The bacterial injectisome, or type III secretion system (T3SS), is a specialized syringe-shaped protein-export system utilized by many pathogenic Gram-negative bacteria for the injection of virulence proteins (effectors) into host cells. The injectisome can be divided into three major regions: the inner- (IM) and outer-membrane (OM) spanning basal body with associated export apparatus and ATPase components, an extracellular needle, and a terminating pore inserted into the host cell membrane called the translocon. The major structural scaffold of the basal body is comprised largely of three proteins that arrange into a series of highly oligomerized, concentric rings: two intimately associated proteins localized to the IM - PrgK/EscJ/MxiJ and PrgH/EscD/MxiG, and a third protein belonging to the secretin family of OM proteins, InvG/EscC/MxiD (Salmonella enterica serovar Typhimurium SPI-1, Enteropathogenic Escherichia coli (EPEC) LEE and Shigella dysenteriae nomenclature, respectively). In summary, we report the crystal structures for the cytoplasmic and periplasmic domains of PrgH and InvG, two of the main basal body components of the prototypical Salmonella SPI-1 injectisome.

Superposition of the InvG and EscC crystal structures revealed a similar organization, with the N0 and N1 domains common to the secretin family; however, the relative orientation of these domains is shifted 36 degrees between the two proteins. Similarly, a dimer formed by a unit cell translation from the InvG crystal lattice superposes with a dimer from the modelled 15-mer ring. Collectively, the crystallographic packing interfaces we observe support and mirror the low energy interfaces generated in our modelled basal body. This would be consistent with a model whereby the soluble domains have low-affinity interaction surfaces for oligomerization, which can be captured by the high concentration in the crystallization experiment. Finally, for InvG we observed a loop (residues 95–99) forming a series of side-chain contacts with the adjacent subunit. Mutation of Gln97 within the loop (which forms a hydrogen bond with the adjacent molecule) to leucine – but not alanine - abrogates secretion (top). Mutation to alanine of the strictly conserved Asp95 within the loop (which lacks any direct interactions with the neighbouring protomer) has no effect on secretion. Furthermore, we observed a positively charged interior collar of the InvG ring corresponding to the N0 domain, where residues are proposed to be in contact with the inner rod and socket. This surface is formed by a set of basic residues lying on one side of the InvG monomer. In particular, we have previously shown that mutation of Lys67 abrogates secretion by altering substrate switching.

> GSGYSSEKIPVTGSGFVAKDDSLRTFFDAMALQLKEPVIVSKMAARKKITGNFEFHDPNALLEKLSLQLGLIWYFDGQAIYIYDASEMRNAVVSLRNVSLNEFNNFLKRSGLYNKNYPLRGDNRKGTFYVSGPPVYVDMVVNAATMMDKQNDGIELGRQ The IE gene product, infected cell protein 4 (ICP4) is a transcriptional regulator with a prominent role within this cascade. ICP4 can induce the expression of E and L genes, while conversely it can act as a repressor notably of itself and also other IE genes. ICP4 homo-dimerization is mediated by the DBD, this region interacts preferentially with a bi-partite and asymmetric DNA consensus sequence RTCGTCnnYnYSG (where R is a purine, Y is a pyrimidine, S is a C or G and n is any base). Here we present the crystal structure of the functionally essential ICP4 DNA binding domain in complex with a segment from its own promoter, revealing a novel homo-dimeric fold.

The combination of the ICP4 DBD, residues 258–487 (ICP4N) with a 19mer DNA duplex matching the consensus site from the ICP4 promoter (IE3_19mer), resulted in the formation of a stoichiometric complex, which can be readily separated by gel filtration. It was also possible to form a smaller ICP4:DNA complex using a combination of truncated ICP4 DBD, residues 288–487 (ICP4NΔIDR), which eliminated a predicted IDR, mixed with a shorter 12mer duplex (IE3_12mer). Superposition of the truncated ICP4NΔIDR polypeptides with ICP4N (chains C and D) indicated no global conformational changes and a backbone RMSD of 0.8 Å for aa301–484. However there were some local structural differences. In particular the S-loop in chain B of ICP4NΔIDR is in a different conformation and lacks clear electron density for residues 412–418, and also the associated 12mer DNA is notably shifted compared to the 19mer DNA, with an RMSD of 1.6 Å. The ICP4NΔIDR·IE3_12mer data therefore indicated that the isolated globular domain can bind to a segment of the ICP4 consensus DNA sequence, but with some local structural readjustments, in comparison to the ICP4N·IE3_19mer structure which contains the complete DBD and whole consensus sequence. Characterization of ICP4 in solution by analytical ultracentrifugation (AUC) and SEC-MALS exclusively detected an ICP4N homodimer in the presence and absence of DNA, and the truncated construct aa288–485 (ICP4NΔIDR) was also a homodimer. In comparison, the affinity of the shorter ICP4ΔIDR construct (aa288–487) for both WT and mutant DNA was three orders of magnitude weaker relative to that measured for ICP4N·WT. These results suggest that an absolute requirement for tight specific binding is the presence of the intrinsically disordered N-terminal region, whereas if this region is deleted, the affinity for DNA consensus sequence is not only reduced, but approximately half of this consensus sequence is no longer recognized.

>GPRRVELDADATSGAFYARYRDGYVSGEPWPGAGPPPPGRVLYGGLGDSRPGLWGAPEAEEARRRFEASGAPAAVWAPELGDAAQQYALITRLLYTPDAEAMGWLQNPRVVPGDVALDQACFRISGAARNSSSFITGSVARAVPHLGYAMAAGRFGWGLAHAAAAVAMSRRYDRAQKGFLLTSLRRAYAPLLARENAALTG[2x]>[3x]MTTPSRRRLMRDFKKLQEDPPAGVSGAPTEDNILTWEAIIFGPQETPFEDGTFKLSLEFTEEYPNKPPTVKFISKMFH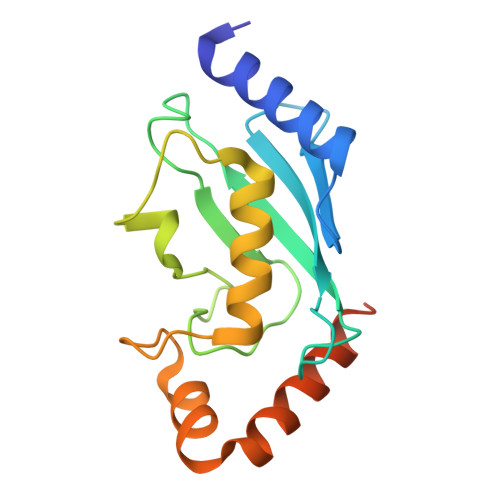PNVYADGSICLDILQNRWSPTYDVAAILTSIQSLLDEPNPNSPANSLAAQLYQENRREYEKRVQQIVEQSWLNFGENEGDAVLKD>[2x]MTETDFKLKYWGNQEQDYILPTVG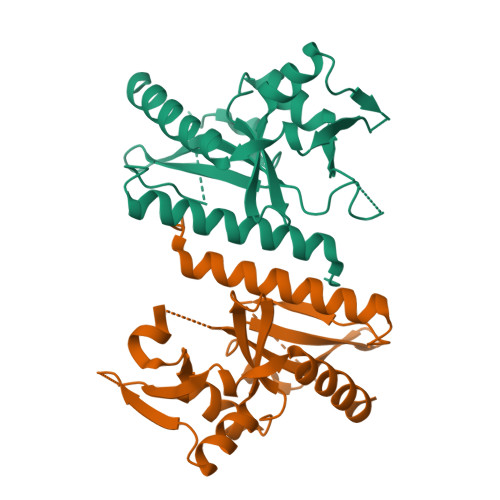LGREYLVLGKLLISLSKWRAKGLIDFDVYLRPTGVGTLTNTINYEYYKGLEDKYDLTLYIRAKDSYYPLLWIDITGSSWTEEQSKERYGESIYAILSVKVETAKKYDVLGRVFFIHYNDTEDKLKCISALQILNLERQNKIKKDKFERGAKSEYYLIPTSYWKNLTELRIALRGFYQSFKEYLARSNK>[12x]PSMMPQWSYMHISGQDASEYLSPGLVQFARATETYFSLNNKFRNPTVAPTHDVTTDRSQRLTLRFIPVDREDTAYSYKARFTLAVGDNRVLDMASTYFDIRGVLDRGPTFKPYSGTAYNALAPKGAPNPCEWDEAATALEINLEEEDDDNEDEVDEQAEQQKTHVFGQAPYSGINITKEGIQIGVEGQTPKYADKTFQPEPQIGESQWYETEINHAAGRVLKKTTPMKPCYGSYAKPTNENGGQGILVKQQNGKLESQVEMQFFSTTEATAGNGDNLTPKVVLYSEDVDIETPDTHISYMPTIKEGNSRELMGQQSMPNRPNYIAFRDNFIGLMYYNSTGNMGVLAGQASQLNAVVDLQDRNTELSYQLLLDSIGDRTRYFSMWNQAVDSYDPDVRIIENHGTEDELPNYCFPLGGVINTETLTKVKPKTGQENGWEKDATEFSDKNEIRVGNNFAMEINLNANLWRNFLYSNIALYLPDKLKYSPSNVKISDNPNTYDYMNKRVVAPGLVDCYINLGARWSLDYMDNVNPFNHHRNAGLRYRSMLLGNGRYVPFHIQVPQKFFAIKNLLLLPGSYTYEWNFRKDVNMVLQSSLGNDLRVDGASIKFDSICLYATFFPMAHNTASTLEAMLRNDTNDQSFNDYLSAANMLYPIPANATNVPISIPSRNWAAFRGWAFTRLKTKETPSLGSGYDPYYTYSGSIPYLDGTFYLNHTFKKVAITFDSSVSWPGNDRLLTPNEFEIKRSVDGEGYNVAQCNMTKDWFLVQMLANYNIGYQGFYIPESYKDRMYSFFRNFQPMSRQVVDDTKYKDYQQVGILHQHNNSGFVGYLAPTMREGQAYPANFPYPLIGKTAVDSITQKKFLCDRTLWRIPFSSNFMSMGALTDLGQNLLYANSAHALDMTFEVDPMDEPTLLYVLFEVFDVVRVHRPHRGVIETVYLRTPFSAGNATT;> MMQDATDPAVRAALQSQPSGLNSTDDWRQVMDRIMSLTARNPDAFRQQPQANRLSAILEAVVPARANPTHEKVLAIVNALAENRAIRPDEAGLVYDALLQRVARYNSGNVQTNLDRLVGDVREAVAQRERAQQQGNLGSMVALNAFLSTQPANVPRGQEDYTNFVSALRLMVTETPQSEVYQSGPDYFFQTSRQGLQTVNLSQAFKNLQGLWGVRAPTGDRATVSSLLTPNSRLLLLLIAPFTDSGS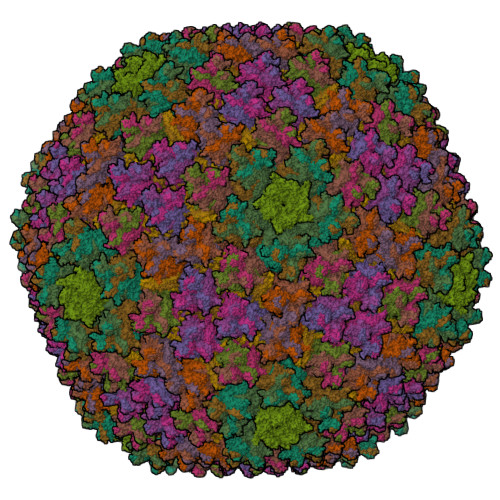VSRDTYLGHLLTLYREAIGQAHVDEHTFQEITSVSRALGQEDTGSLEATLNYLLTNRRQKIPSLHSLNSEEERILRYVQQSVSLNLMRDGVTPSVALDMTARNMEPGMYASNRPFINRLMDYLHRAAAVNPEYFTNAILNPHWLPPPGFYTGGFEVPEGNDGFLWDDIDDSVFSPQPQTLLELQQREQAEAALRKESFRRPSSLSDLGAAAPRSDASSPFPSLIGSLTSTRTTRPRLLGEEEYLNNSLLQPQREKNLPPAFPNNGIESLVDKMSRWKTYAQEHRDVPGPRPPTRRQRHDRQRGLVWEDDDSADDSSVLDLGGSGNPFAHLRPRLGRMF;> MRRAAMYEEGPPPSYESVVSAAPVAAALGSPFDAPLDPPFVPPRYLRPTGGRNSIRYSELAPLFDTTRVYLVDNKSTDVASLNYQNDHSNFLTTVIQNNDYSPGEASTQTINLDDRSHWGGDLKTILHTNMPNVNEFMFTNKFKARVMVSRLPTKDNQVELKYEWVEFTLPEGNYSETMTIDLMNNAIVEHYLKVGRQNGVLESDIGVKFDTRNFRLGFDPVTGLVMPGVYTNEAFHPDIILLPGCGVDFTHSRLSNLLGIRKRQPFQEGFRITYDDLEGGNIPALLDVDAYQASLKDDTEQGGGGAGGSNSSGSGAEENSNAAAAAMQPVEDMNDHAIRGDTFATRAEEKRAEAEAAAEAAAPAAQPEVEKPQKKPVIKPLTEDSKKRSYNLISNDSTFTQYRSWYLAYNYGDPQTGIRSWTLLCTPDVTCGSEQVYWSLPDMMQDPVTFRSTRQISNFPVVGAELLPVHSKSFYNDQAVYSQLIRQFTSLTHVFNRFPENQILARPPAPTITTVSENVPALTDHGTLPLRNSIGGVQRVTITDARRRTCPYVYKALGIVSPRVLSSRTF;>[4x]MSTNSFDGSIVSSYLTTRMPPWAGVRQNVMGSSIDGRPVLPANSTTLTYETVSGTPLETAASAAASAAAATARGIVTDFAFLSPLASSAASRSSARDDKLTALLAQLDSLTRELNVVSQQLLDLRQQVSALKASSPPNAV;>MSKEIPTPYMWSYQPQMGLAAGAAQDYSTRINYMSAGPHMISRVNGIRAHRNRILLEQAAITTTPRNNLNPRSWPAALVYQESPAPTTVVLPRDAQAEVQMTNSGAQLAGGFRHRVRSPGQGITHLTIRGRGIQLNDESVSSSLGLRPDGTFQIGGAGRPSFTPRQAILTLQTSSSEPRSGGIGTLQFIEEFVPSVYFNPFSGPPGHYPDQFIPNFDAVKDSADGYD[2x];> FASLAPRHGSRPFMGNWQDIGTSN>[2x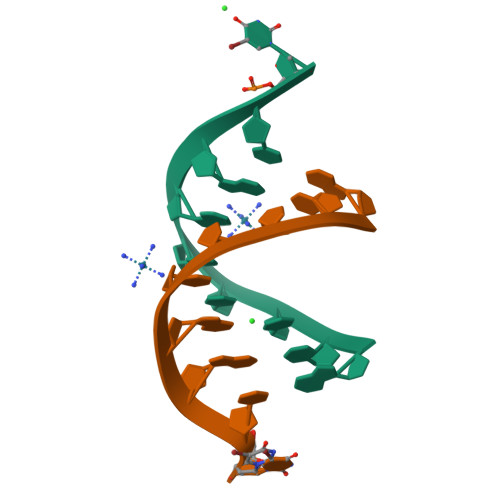]GCUUCGGCU> SMQRTVARDITLLECVGKGRYGEVWRGSWQGENVAVKIFSSRDEKSWFRETELYNTVMLRHENILGFIASDMTSRHSSTQLWLITHYHEMGSLYDYLQLTTLDTVSCLRIVLSIASGLAHLHIEIFGTQGKPAIAHRDLKSKNILVKKNGQCCIADLGLAVMHSQSTNQLDVGNNPRVGTKRYMAPEVLDET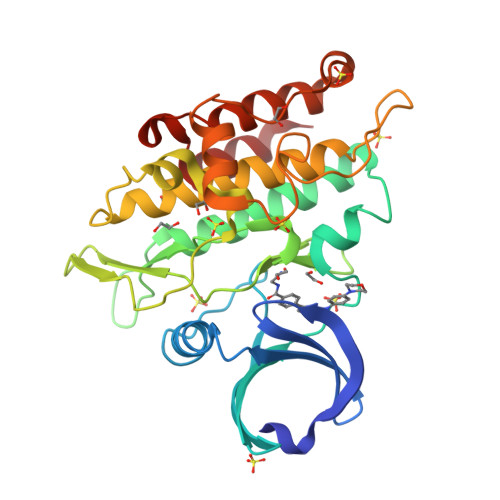IQVDCFDSYKRVDIWAFGLVLWEVARRMVSNGIVEDYKPPFYDVVPNDPSFEDMRKVVCVDQQRPNIPNRWFSDPTLTSLAKLMKECWYQNPSARLTALRIKKTLTKID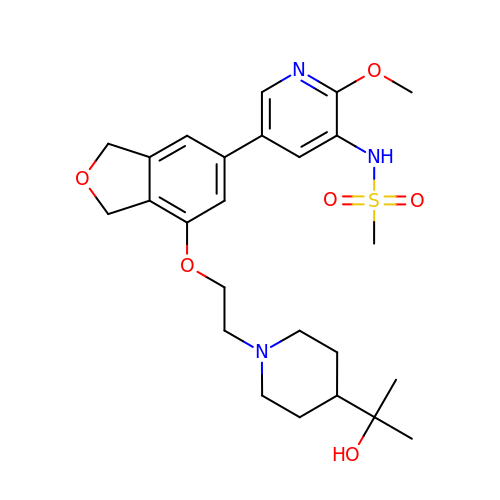~{N}-[2-methoxy-5-[7-[2-[4-(2-oxidanylpropan-2-yl)piperidin-1-yl]ethoxy]-1,3-dihydro-2-benzofuran-5-yl]pyridin-3-yl]methanesulfonamide | C25 H35 N3 O6 S | YTBODSVQSOILIJ-UHFFFAOYSA-N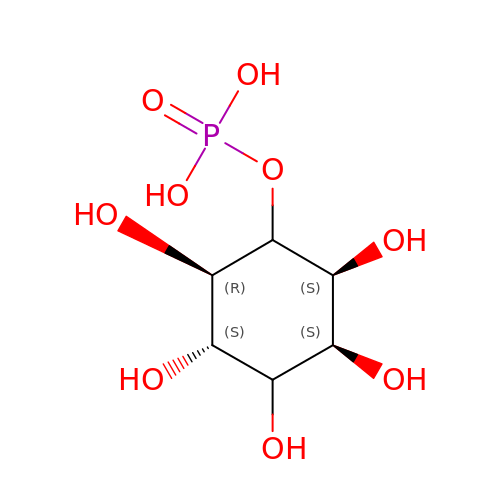D-MYO-INOSITOL-4-PHOSPHATE | C6 H13 O9 P | INAPMGSXUVUWAF-CNWJWELYSA-N> KLP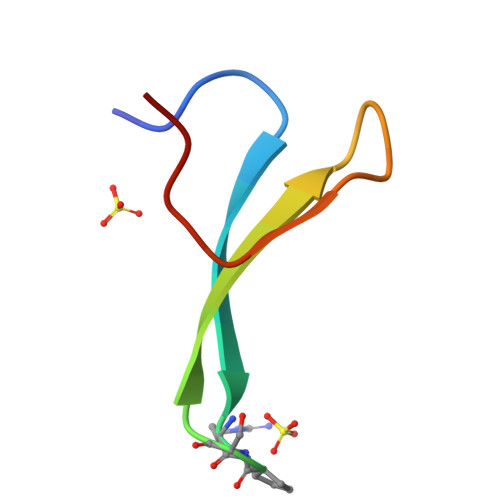PGWEKRMSRXSGRVYYFNHITNASQWERPSG> GYWGYQEFLDEFPEQRNLTNALSEAVRAQPVPLSKPTQRPIKISVVYPGQQVSDYWVRNIASFEKRLYKLNINYQLN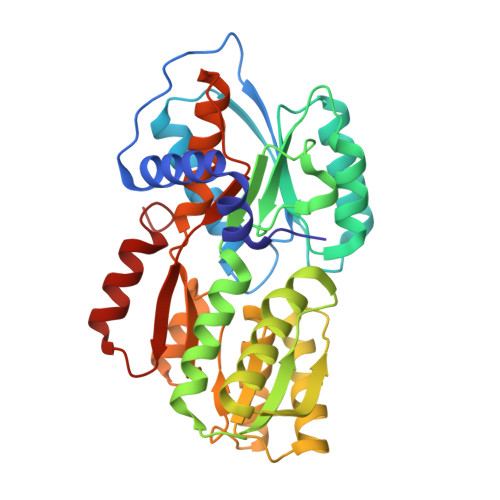QVFTRPNADIKQQSLSLMEALKSKSDYLIFTLDTTRHRKFVEHVLDSTNTKLILQNITTPVREWDKHQPFLYVGFDHAEGSRELATEFGKFFPKHTYYSVLYFSEGYISDVRGDTFIHQVNRDNNFELQSAYYTKATKQSGYDAAKASLAKHPDVDFIYACSTDVALGAVDALAELGREDIMINGWGGGSAELDAIQKGDLDITVMRMNDDTGIAMAEAIKWDLEDKPVPTVYSGDFEIVTKADSPERIEALKKRAFRYSDN>GSHMISEPVDIKYLENNQYSDEGIKAYEFIFGEDYISSGGIIATTKILSDIQLDANSKVLDIGSGLGGGCKYI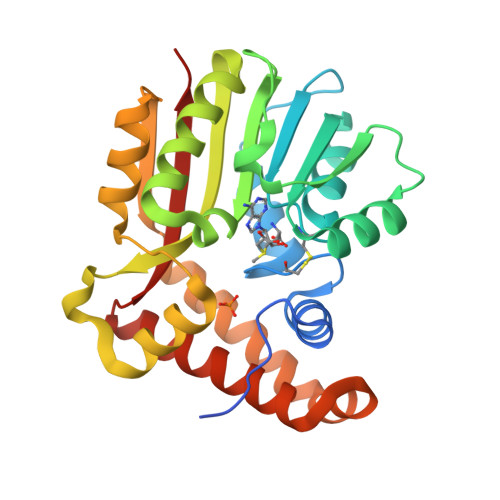NEKYGAHVHGVDICEKMVTIAKLRNQDKAKIEFEAKDILKKDFPESTFDMIYSRDSILHLSYADKKMLFEKCYKWLKPNGILLITDYCADKIENWDEEFKAYIKKRKYTLMPIQEYGDLIKSCKFQNVEAKDISDYWLELLQLELSKLEEKKEEFLKVYSIKEYNSLKDGWTRKIKDTKRDLQKWGYFKAQKMI[2x]>MGLPLMMERSSNNNNVELSRVAVSDTHGEDSPYFAGWKAYDENPYDESHNPSGVIQMGLAENQVSFDLLETYLEKKNPEGSMWGSKGAPGFRENALFQDYHGLKTFRQAMASFMEQIRGGKARFDPDRIVLTAGATAANELLTFILADPNDALLVPTPYYPGFDRDLRWRTGVKIVPIHCDSSNHFQITPEALESAYQTARDANIRVRGVLITNPSNPLGATVQKKVLEDLLDFCVRKNIHLVSDEIYSGSVFHASEFTSVAEIVENIDDVSVKERVHIVYSLSKDLGLPGFRVGTIYSYNDNVVRTARRMSSFTLVSSQTQHMLASMLSDEEFTEKYIRINRERLRRRYDTIVEGLKKAGIECLKGNAGLFCWMNLGFLLEKKTKDGELQLWDVILKELNLNISPGSSCHCSEVGWFRVCFANMSENTLEIALKRIHEFMDRRRRF[4x]

The rate-limiting enzyme of ethylene biosynthesis is 1-aminocyclopropane-1-carboxylate (ACC) synthase (ACS), which is generally believed to be a single-activity enzyme evolving from aspartate aminotransferases. All ACS proteins contain a conserved aspartate aminotransferase (AAT)–like domain and belong to the α superfamily of pyridoxal-5′-phosphate (PLP)–dependent enzymes. AtACS7 is one of the genuine ACS enzymes of ethylene biosynthesis in Arabidopsis, catalyzing the conversion of SAM to ACC through α,γ-elimination (top).

There are four AtACS7-PPG complexes that make up two dimers in each asymmetric unit. The two dimers (chain A and B dimer and chain C and D dimer) exhibit almost identical structures, with a root mean square deviation (RMSD) of 0.76 Å, and both have the classic AAT-like folding. The structures of the two subunits are nearly the same, with an RMSD of 0.44 Å. For the active site, Asn217 and Tyr248 both form hydrogen bonds with the O3 of PPG, and Asp245 forms a hydrogen bond with the N1 of PPG. Arg293 and Arg419 form salt bridges with the carboxyl group and phosphate group of PPG, respectively. Tyr160 exhibits parallel stacking over the pyridine ring of PPG, while the key catalytic residue Lys285 is located at the opposite side of the PPG from Tyr160. In addition to the above residues that belong to the same AtACS7 subunit, the side chain of Gln98 from the other subunit is protruding near the PPG molecule. The overall and the active site structures of the two ACSs are almost identical, with the RMSD (for the Cα atoms) of 0.83 Å in the overall structure comparison and 0.176 Å in the active-site residue comparison. To estimate the role of Q98, SAM-aldimine was docked to the wild-type AtACS7 structure using the program AUTODOCK. The result showed that the amide group of Q98 directly approached the sulfur atom of SAM.> HHHHHHQYDWDNVPIPANAGAGKTWKLQTAASDDFNYTFNPTNNVVDFGPNGNMKWYNKYHNRPNGQPNNFEGPGPTKWMQNHVAVSGG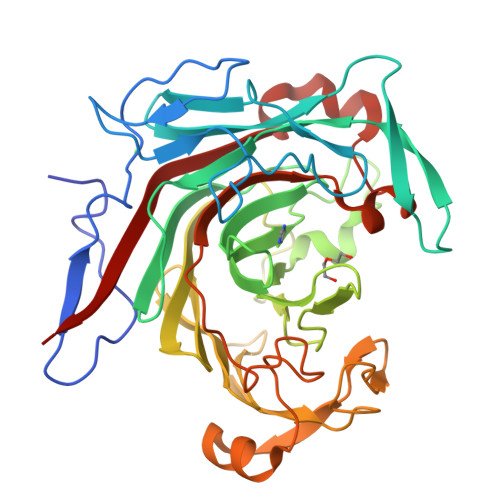NLNIWASRIPGATKSFTGSNNTPISRPETRAGCITNKTRVKYPVFVEARVKVMNSTLASDIWLLSPDDTQEIDIMECYGGPGNDNRNSYFASKIHLSHHVFIRPPNFKDYQPADLNSWWGKNGVTQWGGKTIRIGVNWVSPTRLEYFVDGQMVRILDNDAVQTRLADGTWQYTYPAGVTSTGVNGQLIKENGYQKMNIASSLSDAKNKSNISVIDPFNYLNNGRKFSKEMDIIINVEDQSWQAEAYRSPNAAEMANFYDNNLLVDWIRVYKPVN>[3x]NKNNTHKSNRKGKPVKQPSSHKRNNNPSRSVAPVAKANALRTTSSNSILLKGCD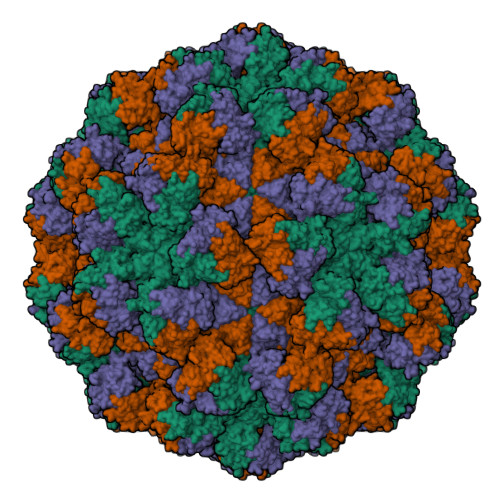RIVTVVDASTYDAGSAIVSIPITPDIAYRLGSTARTFQRIKYRSLKFRVNAQCATTTAGGYVAGFVKDAADVLPTGTASIPYLMSNTGSFTQPWWKSTVHNVKIPQKLFYTEAPTRGADAVREYCPGQFHVLVDSKPSQICPVTVDLEWVVELHDATFRKESDQTAISAIVADHTLNVYGLPATSNRVGHILISPIGQTPKDLTPTRFATFFGFLPDDKFCVRIPTPVDVVLTGDNVYQSVEATHIRAYLVNGGLGIDFHLAAYNDTTHTIQPIIPTLWNVYDVTGAVTAPFTSAIYDNHVWTHKDKFVPVSFQDEPIPGTVFDYLYPRSYSLPSSN>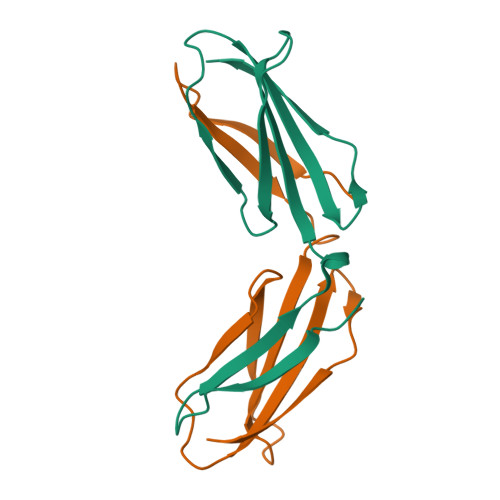[3x]MRLDAPSQIEVKDVTDTTALITWSMQLSQLEGIELTYGIKDVPGDRTTIDLTEDENQYSIGNLKPDTEYEVSLISRRGDMSSNPAKETFTTGLAAALEHHHHHH>[4x]MSLKIKHEHIRMAMNAWAHPDGEKVPAAEITRAYFELGMTFPELYDDSHPE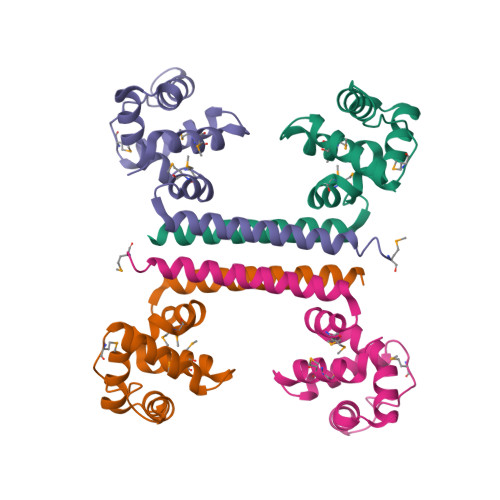ALARNTQKIFRWVEKDTPDAVEKIQALLPAIEKSMPPLLVARMRSHSSAYFRELVETRERLVRDADDFVAVAIAGFNQMNRGGPAGNIVAVHEGHHHHHH GLUTAMOL-AMP | C15 H22 N6 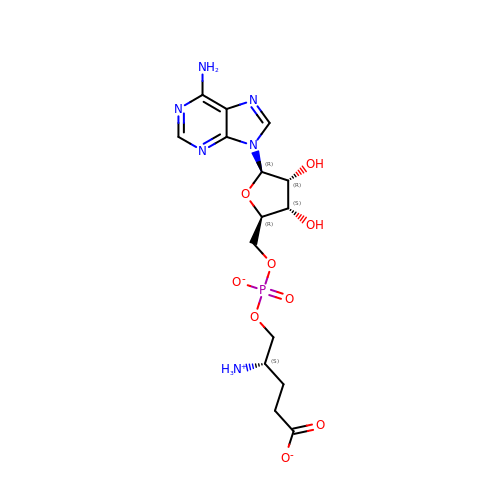O9 P | JDELUWYDJMPPMI-SBZSCLMQSA-M>SNAMPSIRYPSTEFPALTGFTVPIPETWQPDPTMGTQFAARPHTPPQ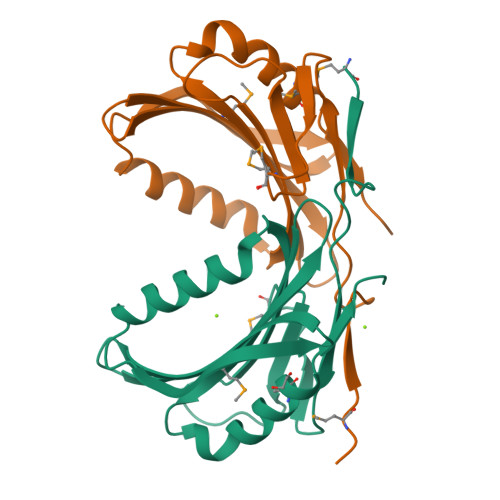GFTPNIIGTVRRAATGALHNQRTELDQRATQLPDYAERGRTETTVDGFPAYHIEYAYRHHGTITIAQMITLVEVSHPHAVDIIQLTATCAGDQTADYWDTFRLMHADLTVQPHG[2x]> MAESKPTPQSTFTGPIVVDPITRIEGHLRIMVEVENGKVKDAWSSSQLFRGLEIILKGRDPRDAQHFTQRACGMCTYVHALASSRCVDDAVKVSIPANARMMRNLVMASQYLHDHLVHFYHLHALDWVDVTAALKADPNKAAKLAASIAPARPGNSAKALKAVQDKLKAFVESGQLGIFTNAYFLGGHKAYYLPPEVDLIAT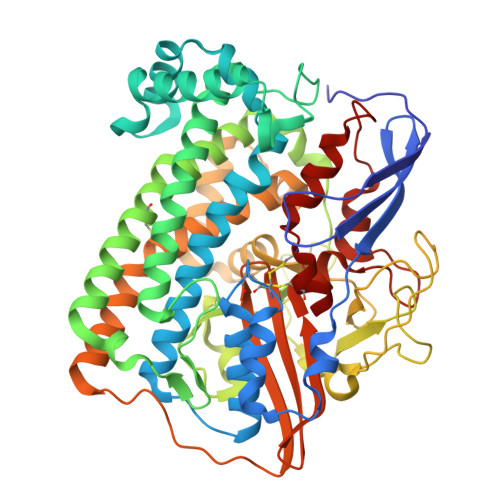AHYLEALHMQVKAASAMAILGGKNPHTQFTVVGGCSNYQGLTKDPLANYLALSKEVCQFVNECYIPDLLAVAGFYKDWGGIGGTSNYLAFGEFATDDSSPEKHLATSQFPSGVITGRDLGKVDNVDLGAIYEDVKYSWYAPGGDGKHPYDGVTDPKYTKLDDKDHYSWMKAPRYKGKAMEVGPLARTFIAYAKGQPDFKKVVDMVLGKLSVPATALHSTLGRTAARGIETAIVCANMEKWIKEMADSGAKDNTLCAKWEMPEESKGVGLADAPRGALSHWIRIKGKKIDNFQLVVPSTWNLGPRGAQGDKSPVEEALIGTPIADPKRPVEILRTVHAFDPCIACGVH> MKNLDCWVDNEEDIDVILKKSTILNLDINNDIISDISGFNSSVITYPDAQLVPGINGKAIHLVNNESSEVIVHKAMDIEYNDMFNNFTVSFWLRVPKVSASHLEQYGTNEYSIISSMKKHSLSIGSGWSVSLKGNNLIWTLKDSAGEVRQITFRDLPDKFNAYLANKWVFITITNDRLSSANLYINGVLMGSAEITGLGAIREDNNITLKLDRCNNNNQYVSIDKFRIFCKALNPKEIEKLYTSYLSITFLRDFWGNPLRYDTEYYLIPVASSSKDVQLKNITDYMYLTNAPSYTNGKLNIYYRRLYNGLKFIIKRYTPNNE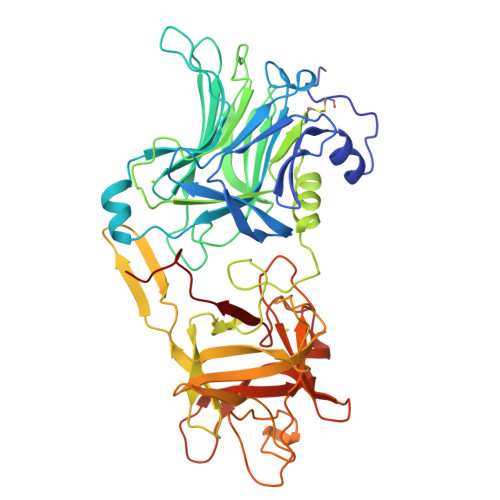IDSFVKSGDFIKLYVSYNNNEHIVGYPKDGNAFNNLDRILRVGYNAPGIPLYKKMEAVKLRDLKTYSVQLKLYDDKNASLGLVGTHNGQIGNDPNRDILIASNWYFNHLKDKILGCDWYFVPTDEGWTND>MGSSHHHHHHSSGENLYFQGHMAILKLGNRGSEVKSLQQSLNKIGFSLVADGIFGKATENAVKSVQAGAGLVIDGIAGPKTFYAIRNAGDAHQEHLTEADLVD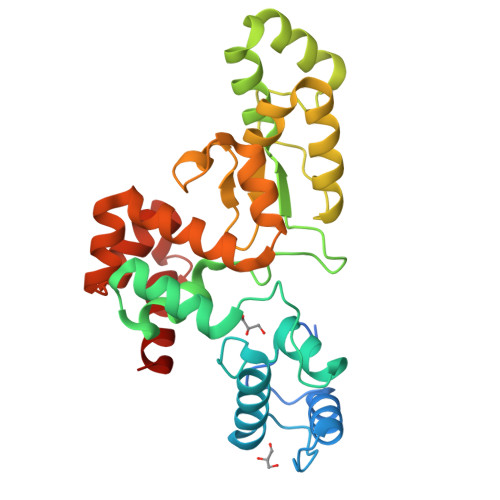AARELGVELASMKAVNQVESRGTGFTKTGKIKTLFERHIMYKKVAAKFGQARANALYQLYPTLVNPNSGGYIGGDAELERLQGAIALDEDCAYESASYGLFQIMGFNCQICGYPNAKEMFTDFLTGERAHLLAFVKFIKADANMWKALKNKNWAEFARRYNGPAYAKNQYDTKLAAAYKSFC[2x]> MSRVQLALRVPDLEASIGFYSKLFGTGPAKVRPGYANFAIAEPPLKLVLIEGAGEDATRLDHLGVEVEDSAQVGHAARRLKESGLATVEENDTACCYAVQDKVWVTG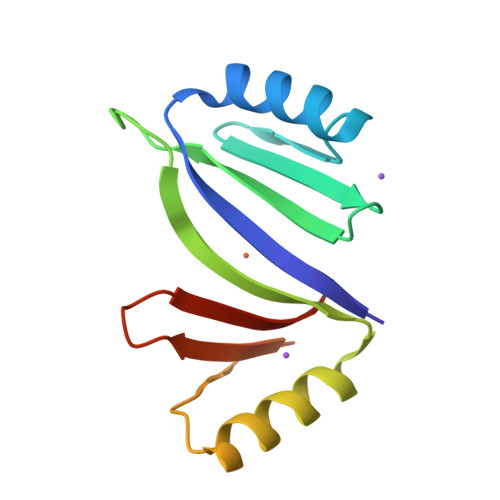PGGEPWEVYVVKGDAD>[2x]GSDRPTPVPLPNSEQFYLENDRGEPYLIQVSWPLHWEDKQTGRGPLPIIYIVDGNALFLTATEAAWRRAAASHFAGGGIIVAIGYPLKGKLYDARRRSFDLTPPTACAPVGYGGADVFLDFIENSVRPAVQARFPQVSLAREALYGHAYGGLLALHALFTRPQSFDCYIASSPSIW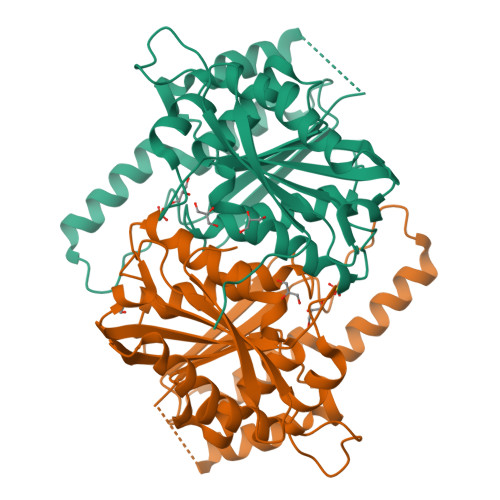WNSLCILHEAKAFVETKKVSHDQSPSLMVSWGSWEQHPPRWADELLDHYEARKRTAAELRMADNALDLCAMLHGCSRLHALIKTEYEGEDHTSVMSCSVSRGLTMFFEDWPFHQSG(2'R,3R,4'R,5'R)-6-chloro-4'-(3-chloro-2-fluorophenyl)-2'-(2,2-dimethylpropyl)-N-(2-morpholin-4-ylethyl)-2-oxo-1,2-dihydrospiro[indole-3,3'-pyrrolidine]-5'-carboxamide | C29 H35 Cl2 F N4 O3 | 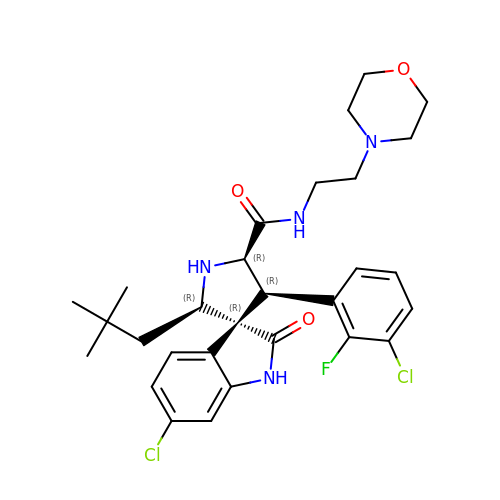YTBYOWZWBDYLQF-BYHVZLFPSA-N>AHHHHHHSSGLVPRGSHMANKAVNDFILAMNYDKKKLLTHQGESIENRFIKEGNQLPDEFVVIERKKRSLSTNTSDISVTATNDSRLYPGALLVVDETLLENNPTLLAVDRAPMTYSIDLPGLASSDSFLQVEDPSNSSVRGAVNDLLAKWHQDYGQVNNVPARMQYEKITAHSMEQLKVKFGSAFEKTGNSLDIDFNSVHSGEKQIQIVNFKQIYYTVSVDAVKNPGDVFQDTVTVEDLKQRGISAERPLVYISSVAYGRQVYLKLETTSKSDEVEAAFEALIKGVKVAPQTEWKQILDNTEVKAVILGGDPSSGARVVTGKVDMVEDLIQEGSRFTADHPGLPISYTTSFLRDNVVATFQNSTDYVETKVTAYRNGDLLLDHSGAYV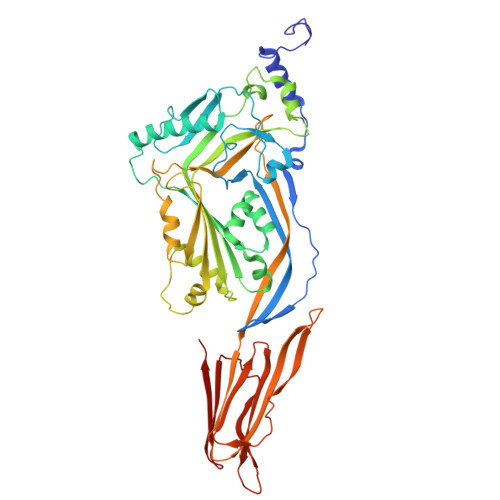AQYYITWDELSYDHQGKEVLTPKAWDRNGQDLTAHFTTSIPLKGNVRNLSVKIRECTGLAWEWWRTVYEKTDLPLVRKRTISIWGTTLYPQVEDKVEND[2x]> MRLSYEALEWRTPIENSTEPVSLPPPPPFFGQERAREALELAIRGGFHAYLVGPPSLGKHEALLAYLSTQSVETPPDLLYVPLSERKVAVLTLPSGQEIHLAEAVEGLLLEVNRLDELFRQGSFLREKTQLEARFKEAREQQLEALRREAQEAGFALSTNGERLELTGPGPVPAELSARLEEVTLGSLAASAELEVALRRLRRDWALHYLNNRFEPLFQRFPQARAYLEALRARLARYAETGEPLDPAQWRPNLLTSSSSGTPPPIVYEPYATAPRLFGRLDYLVDRGVWSTNVSLIRPGAVHRAQGGYLILDALSLKREGTWEAFKRALRNGQVEPVTEPQAPAGLEVEPFPIQMQVILVGTPEAFEGLEEDPAFSELFRIRAEFSPTLPASPENCTALGGWLLAQGFQLTQGGLTRLYDEARRMAEQRDRMDARLVEIRALAEEAAVLGGGLLTAESVEQAIAAREHRSFLSEEEFLRAVQEGVIRLRTTGRAVGEVNSL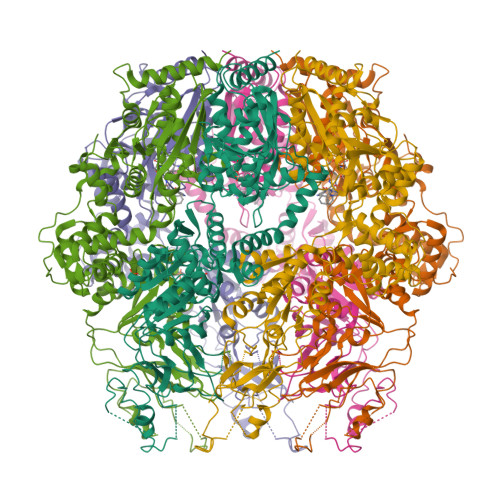VVVEAAPYWGRPARLTARAAPGRDHLISIDREAGLGGQIFHKAVLTLAGYLRSRYIEHGSLPVTISLAFEQNYVSIEGDSAGLAELVAALSAIGNLPLRQDLAVTGAVDQTGKVLAVGAINAKVEGFFRVCKALGLSGTQGVILPEANLANLTLRAEVLEAVRAGQFHIYAVETAEQALEILAGARMEGFRGLQEKIRAGLEAFARLEEGHDKEDREKLAAALEHHHHHH> GPGGDLHMDALLTKFNEDRSLQDENLSQPRTRVRIVDDNLYNKSNPFQLCYKKRDYGSQYYHIYQYRLKTFRERVLKECDKRWDAGFTLNGQLVLKKDKVLDIQGNQPCWCVGSIYCEMKYKPNVLDEVINDTYGAPDLTKSYTDKEGGSDEIMLEDESGRVLLVGDFIRSTPFITGVVVGILGMEAEAGTFQVLDICYPTPLPQNPFPAPIATCPTRGKIALVSGLNLNNTSPDRLLRLEILREFLMGRINNKIDDISLIGRLLICGNSVDFDIKSVNKDELMISLTEFSKFLHNILPSISVDIMPGTNDPSDKSLPQQPFHKSLFDKSLESYFNGSNKEILNLVTNPYEFSYNGVDVLAVSGKNINDICKYVIPSNDNGESENKVEEGESNDFKDDIEHRLDLMECTMKWQNIAP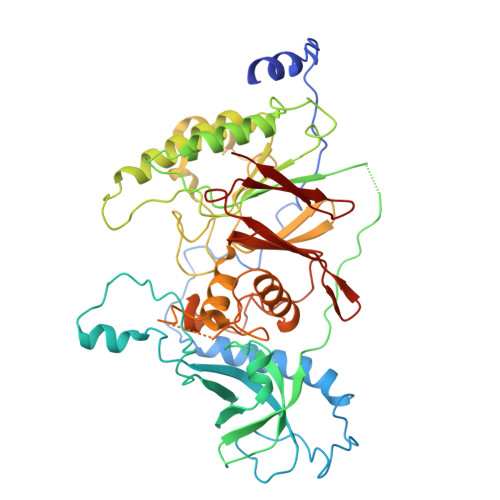TAPDTLWCYPYTDKDPFVLDKWPHVYIVANQPYFGTRVVEIGGKNIKIISVPEFSSTGMIILLDLETLEAETVKIDI> ADPLGCDLPQNHGLLSRNTLVLLHQMRRISPFLCLKDRRDFRF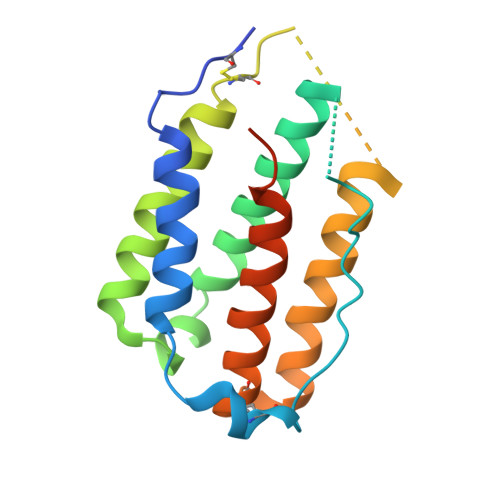PQEMVKGSQLQKAHVMSVLHEMLQQIFSLFHTERSSAAWQMTLLDQLHTGLHQQLQHLETCLLQVVGEGESAGAISSPALTLRRYFQGIRVYLKEKKYSDCAWEVVRMEIMKSLFLSTNMQERLRSKDRDLGSS> GSVGPKTGEENQVLVPNLNPTPENLEVVGDGFKITSSINLVGEEEADENAVNALREFLTANNIEINSENDPNSTTLIIGEVDDDIPELDEALNGTTAENLKEEGYALVSNDGKIAIEGKDGDGTFYGVQTFKQLVKESNIPEVNITDYPTVSARGIVEGFYGTPWTHQDRLDQIKFYGENKLNTYIYAPKDDPYHREKWREPYPESEMQRMQELINASAENKVDFVFGISPGIDIRFDGDAGEEDFNHLITKAESLYDMGVRSFAIYWDDIQDKSAAKHAQVLNRFNEEFVKAKGDVKPLITVPTEY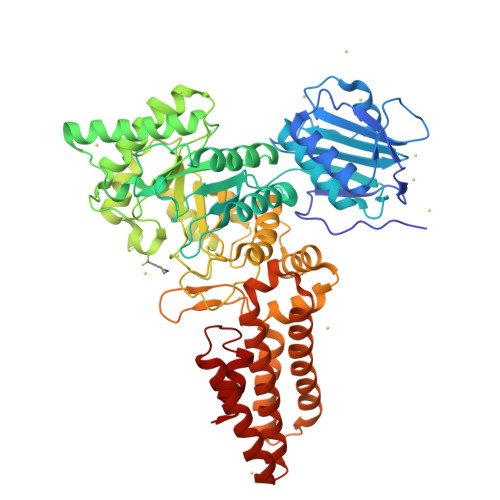DTGAMVSNGQPRAYTRIFAETVDPSIEVMWTGPGVVTNEIPLSDAQLISGIYDRNMAVWWNYPVTDYFKGKLALGPMHGLDKGLNQYVDFFTVNPMEHAELSKISIHTAADYSWNMDNYDYDKAWNRAIDMLYGDLAEDMKVFANHSTRMDNKTWAKSGREDAPELRAKMDELWNKLSSKEDASALIEELYGEFARMEEACNNLKANLPEVALEECSRQLDELITLAQGDKASLDMIVAQLNEDTEAYESAKEIAQNKLNTALSSFAVISEKVAQSFIQEALS>[4x]SNAMTSVAAKHAKGKKLKDVIFVTAGQAQADAKENGRENVVNGTLGAIHDEEGNLVFLKTVKEEYLSLSDSEHVGYAPIAGIPDFLCAAEKECFGNFRPEGHIRSIATAGGTGGIHHLIHNYTEPGDEVLTADWYWGAYRVICSDTGRTLVTYSLFDEHNNFNHEAFQNRVNELAAKQTNVVVIFNTPGNNPTGYSIEDKDWDSILNFLKDLVAIGRNNVIIGIDVAYLDYSGEKDEVRAFFNKFSHL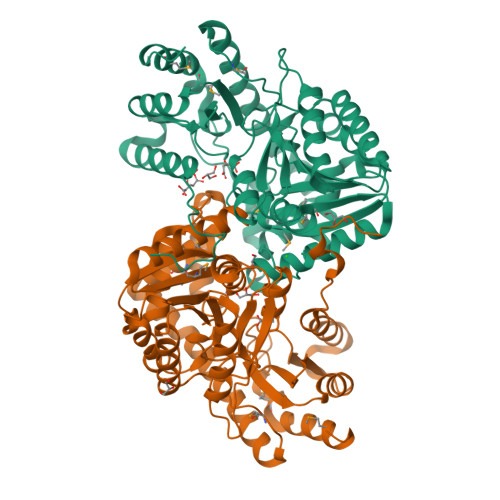PKEILTCVCYSLSKGFTMYGQRVGAMIGISDDEEIADEFFEVNKSTSRATWSNICRPAMRTMANIVADPAKFKEYEAERNCYYQLIRDRADIFKQEAAQVGLPMLPYRGGFFITIPTDSANAICEELKKEHIYVIALANGIRIAACGIPKCQMTGLAEKIYNAMKSLGKL~{N}-oxidanyl-1-phenyl-1,2,3-triazole-4-carboxamide 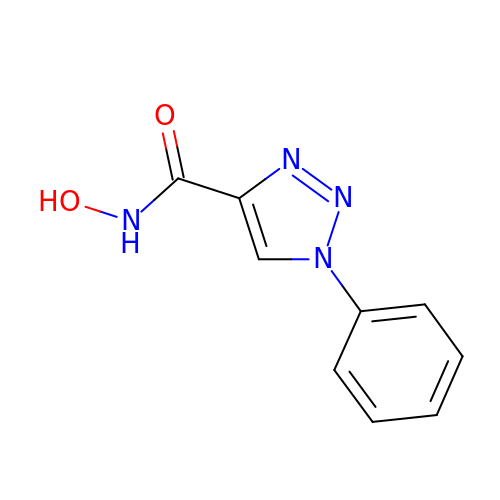| C9 H8 N4 O2 | ALZYWLPUOFGSEC-UHFFFAOYSA-N> ASMTGNECPELQPPVHGKIEPSQAKYFFKDQVLVSCDTGYKVLKDNVEMDTFQIECLKDGTWSNKIPTCKIVDCRAPGELEHGLITFSTRNNLTTYKS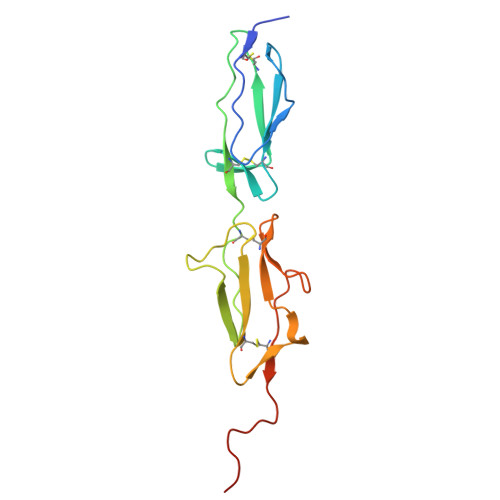EIKYSCQEPYYKMLNNNTGIYTCSAQGVWMNKVLGRSLPTCLPVCGLPKFSRKLMAR>[7x]MTIAIRQLQTHFVGQVSGLDLRKPLTPGEAREVESAMDKYAVLVFHDQDITDEQQMAFALNFGQREDARGGTVTKEKDYRLQSGLNDVSNLGKDGKPLAKDSRTHLFNLGNCLWHSDSSFRPIPAKFSLLSARVVNPTGGNTEFADMRAAYDALDDETKAEIEDLVCEHSLMYSRGSLGFTEYTDEEKQMFKPVLQ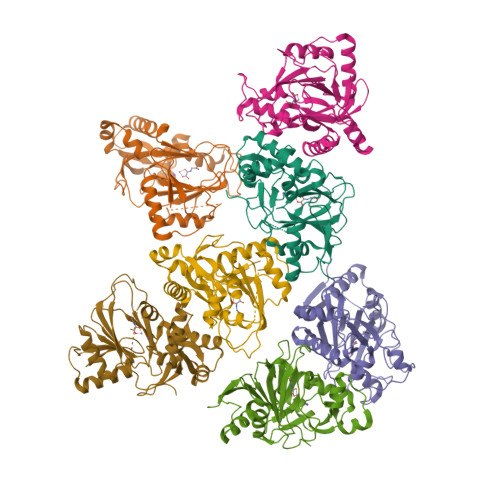RLVRTHPVHRRKSLYLSSHAGKIASMSVPEGRLLLRDLNEHATQPEFVYVHKWKLHDLVMWDNRQTMHRVRRYDQSQPRDMRRATVAGTEPTVQQQAAE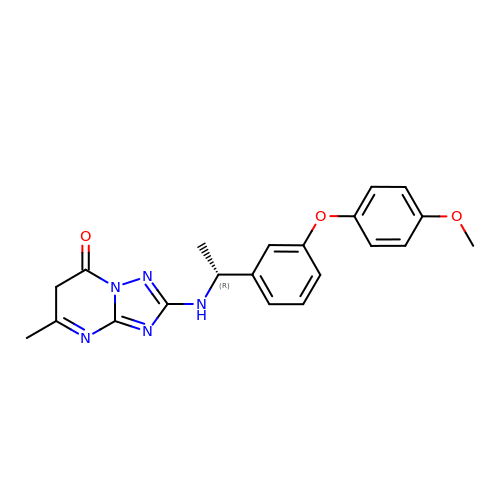2-({(1R)-1-[3-(4-methoxyphenoxy)phenyl]ethyl}amino)-5-methyl[1,2,4]triazolo[1,5-a]pyrimidin-7(6H)-one | C21 H21 N5 O3 | URYYGXLOJAHXGW-CQSZACIVSA-N>[2x]G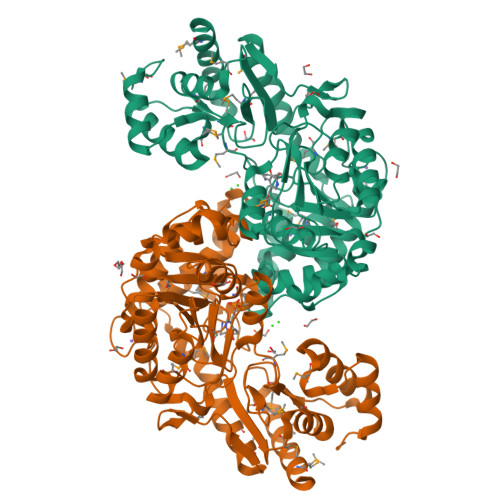MNFPIDEKLIREKQNELHIKDLGMASIRDLVALVTNLEKATGTKFCRMEMGVPGLPAPQIGIETEIQKLREGVASIYPNLDGLPELKQEASRFAKLFVNIDIPARACVPTVGSMQGCFVSFLVANRTHKNREYGTLFIDPGFNLNKLQCRILGQKFESFDLFEYRGEKLREKLESYLQTGQFCSIIYSNPNNPTWQCMTDEELRIIGELATKHDVIVIEDLAYFGMDFRKDYSHPGEPLYQPSVANYTDNYILALSSSKAFSYAGQRIGVLMISGKLYEREYPDLEESFGRLRFGEALSSSALYALSSGATHSAQWGMAAMLKACNDGEYNFRDSVIEYGRKARIMKKMFLDNGFNIVYDKDGNEPLADGFYFTVGYKGMDSSKLIEKFVRYGMCAITLKTTGSKRNEAMRICTSLLPESQFPDLEKRLQMLNAEG> F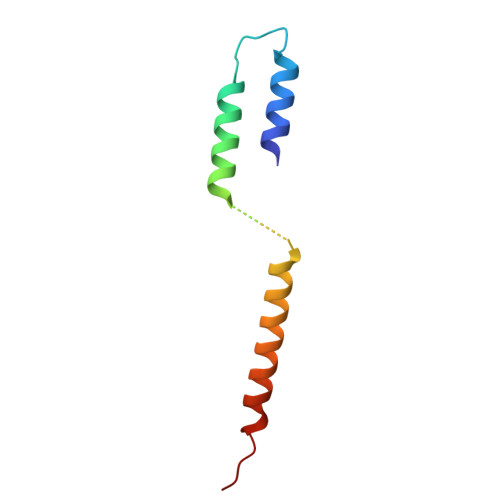LPLVHNVIKCMDKDSPDLHQDLNALKTKFQELRKLIGTMPGIHVSPEQQQQQLHSLREQVRTKNELLQKYKSLCM Furthermore, GDSL-hydrolases are characterised by a three-layered α/β/α-fold with a conserved core structure consisting of five β-strands and at least four α-helices. The GDSL enzymes have catalytic residues, namely Ser, Gly, Asn and His, located in consensus sequences designated as blocks I, II, III, and V, respectively. In the present work, we show that TesA shows lysophospholipase A (lysoPL A) activity with substrate specificity for medium and long chain lysophospholipids (lysoPLs), which are predominantly present in the bacterial cell membranes.

The crystal structure of TesA has been determined at 1.9 Å resolution. There are two molecules per asymmetric unit which are related by a two-fold noncrystallographic symmetry (NCS) (the root-mean-square difference (rmsd) between NCS related molecules A and B is 0.38 Å or Q=0.984; note: for identical structures Q=1). The monomer atomic model comprises residues 1-180 of the protein (light blue), no electron density was observed for the C-terminal His-tag comprised of residues 181-186. The compact single domain structure is comprised of a central five-stranded β-sheet surrounded by five α-helices and three 310 helices. The structure of TesA confirmed these residues as active site residues located on the top of the solvent exposed substrate binding cleft. Both the positioning and the orientation of the catalytic triad residues at structurally conserved topological sites classify TesA as a typical GDSL hydrolase. Interestingly, the conformation of the respective loop in the apo (i.e. ligand-free) form of the TesA structure is similar to that in the complex of TAP with the substrate OCA, but not to the TAP apo state. Interestingly, a comparative B-factor analysis of TesA and TAP revealed significantly lower values for TesA. The more compact structure and the lower B-factor values clearly indicate pronounced conformational rigidity of TesA. The structural alignment shows the presence of both waters in TesA, in identical spatial positions and with the protein environment comprised primarily of highly conserved residues. Superposition of TesA and TAP revealed a structural diversity in the thioester binding site, where TesA shows significantly lower thioesterase activity.

>[2x]MRALLLSGCLALVLLTQQAAAQTLLVVGDSISAALGLDTSQGWVALLQKRLADEGYDYRVVNASISGDTSAGGLARLPALLAEEKPALVVIELGGNDGLRGMAPAQLQQNLASMAQKARAEGAKVLLLGIQLPPNYGPRYIEAFSRVYGAVAAQEKTALVPFFLEGVGGVQGMMQADGIHPALAAQPRLLENVWPTLKPLLHHHHHH>MVREAGEVVAIVPAAGSGERLAVGVPKAFYQLDGQTLIERAVDGLLDSGVVDTVVVAVPADRTDEARQILGHRAMIVAGGSNRTDTVNLALTVLSGTAEPEFVLVHDAARALTPPALVARVVEALRDGYAAV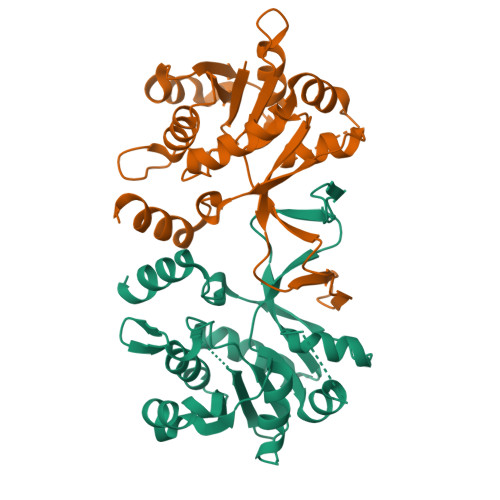VPVLPLSDTIKAVDANGVVLGTPERAGLRAVQTPQGFTTDLLLRSYQRGSLDLPAAEYTDDASLVEHIGGQVQVVDGDPLAFKITTKLDLLLAQAIVRG[4x]>[4x]TTFKIES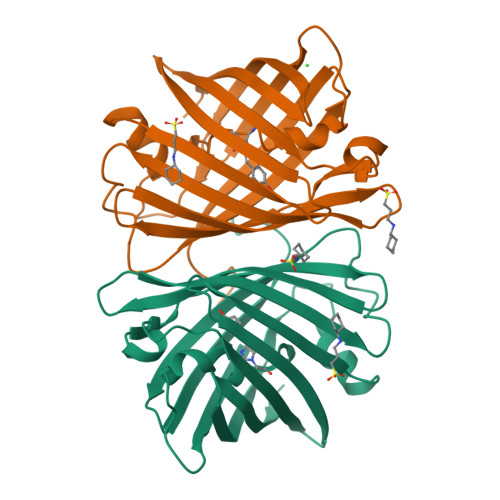RIHGNLNGEKFELVGGGVGEEGRLEIEMKTKDKPLAFSPFLLSTCMGYGFYHFASFPKGTKNIYLHAATNGGYTNTRKEIYEDGGILEVNFRYTYEFNKIIGDVECIGHGFPSQSPIFKDTIVKSCPTVDLMLPMSGNIIASSYARAFQLKDGSFYTAEVKNNIDFKNPIHESFSKSGPMFTHRRVEETHTKENLAMVEYQQVFNSAPRDM> GDRVKKLINSQISLLIGKGLHEFDSLRDPEVNDFRTKMRQFCEEAAAHRQQLGWVEWLQYSFPLQLEPSARGWRAGLLRVSNRALLVNVKFEGSEESFTFQVSTKDMPLALMACALRKKATVFRQPLVEQPEEYALQVNGRHEYLYGNYPLCHFQYICSCLHSGLTPHLTMVHSSSILAMRDEQSNPAPQVQKPRAKPPPIPAKKPSSVSLWSLEQPFSIELIEGRKVNADERMKLVVQAGLFHGNEMLCKTVSSSEVNVCSEPVWKQRLEFDISVCDLPRMARLCFALYAVVEKAKKARSTKKKSKKADCPIAWANLMLFDYKDQLKTGERCLYMWPSVPDEKGELLNPAGTVRGNPNTESAAALVIYLPEVAPHPVYFPALEKILELGRIGERGRITEEEQLQLREILERRGSGELYEHEKDLVWKMRHEVQEHFPEALARLLLVTKWNKHEDVAQMLYLLCSWPELPVLSALELLDFSFPDCYVGSFAIKSLRKLTDDELFQYLLQLVQVLKYESYLDCELTKFLLGRALANRKIGHFLFWHLRSEMHVPSVALRFGLIMEAYCRGSTHHMKVLMKQGEALSKLKALNDFVKVSSQKTTKPQTKEMMHMCMRQETYMEALSHLQSPLDPSTLLEEVCVEQCTFMDSKMKPLWIMYSSEEAGSAGNVGIIFKNGDDLRQDMLTLQMIQLMDVLWKQEGLDLRMTPYGCLPTGDRTGLIEVVLHSDTIANIQLNKSNMAATAAFNKDALLNWLKSKNPGEALDRAIEEFTLSCAGYCVATYVLGIGDRHSDNIMIRESGQLFHIDFGHFLGNFKTKFGINR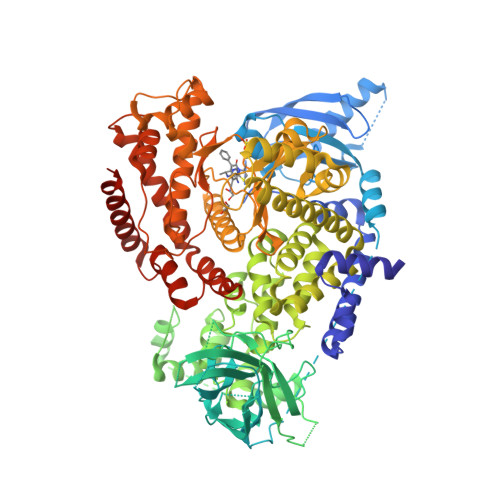ERVPFILTYDFVHVIQQGKTNNSEKFERFRGYCERAYTILRRHGLLFLHLFALMRAAGLPELSCSKDIQYLKDSLALGKTEEEALKHFRVKFNEALRESWKTKVNWLAHNVSKDNRQ>SLWQFGKMINYVMGESGVLQYLSYGCYCGLGGQGQPTDATDRCCFVHDCCYGKVTGCDPKIDSYTYSKKNGDVVCGGDDPCKKQICECDRVATTCFRDNKDTYDIKYWF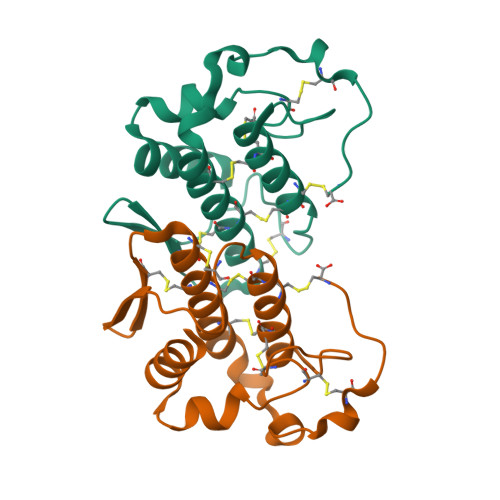YGAKNCQEKSEPC[2x]(3~{R})-3-[(3~{R})-6-fluoranyl-1-oxidanyl-3~{H}-2,1-benzoxaborol-3-yl]-2-methylidene-butanoic acid | C12 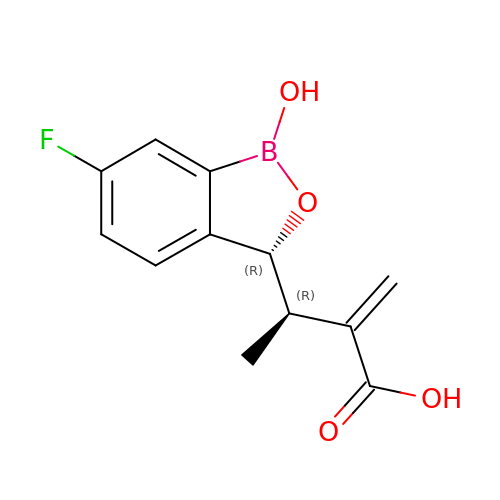H12 B F O4 | PGNFEWJWFZLGLG-KSBSHMNSSA-N>[2x]GSMASLPVLQKESVFQSGAHAYRIPALLYLPGQQSLLAFAEQRASKKDEHAELIVLRRGDYDAPTHQVQWQAQEVVAQARLDGHRSMNPCPLYDAQTGTLFLFFIAIPGQVTQEQQLQTRANVTRLCQVTSTDHGRTWSSPRDLTDAAIGPAYREWSTFAVGPGHCLQLNDRARSLVVPAYAYRKLHPIQRPIPSAFCFLSHDHGRTWARG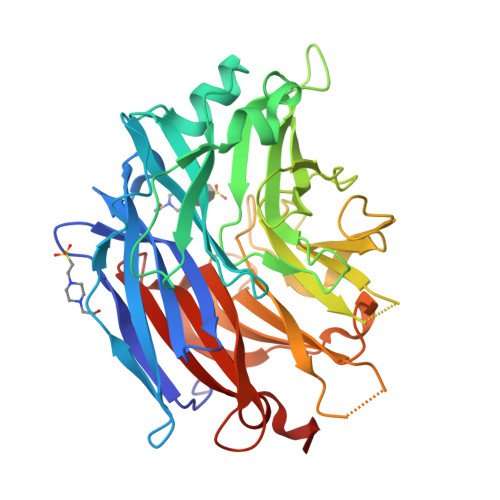HFVAQDTLECQVAEVETGEQRVVTLNARSHLRARVQAQSTNDGLDFQESQLVKKLVEPPPQGCQGSVISFPSPRSGPGSPAQWLLYTHPTHSWQRADLGAYLNPRPPAPEAWSEPVLLAKGSCAYSDLQSMGTGPDGSPLFGCLYEANDYEEIVFLMFTLKQAFPAEYLPQ> QKTGTAEMSSILEERILGADTSVDLEETGRVLSIGDGIARVHGLRNVQAEEMVEFSSGLKGMSLNLEPDNVGVVVFGNDKLIKEGDIVKRTGAIVDVPVGDELLGRVVDALGNAIDGKGPVGSKIRRRVGLKAPGIIPRISVREPMQTGIKAVDSLVPIGRGQRELIIGDRQTGKTSIAIDTIINQKRFNDGTDEKKKLYCIYVAIGQKRSTVAQLVKRLTDADAMKYTIVVSATASDAAPLQYLAPYSGCSMGEYFRDNGKHALIIYDDLSKQAVAYRQMSLLLRRPPGREAYPGDVFYLHSRLLERAAKMNDSFGGGSLTALPVIETQAGDVSAYIPTNVISITDGQIFLETELFYKGIRPAINVGLSVSRVGSAAQTRAMKQVAGTMKLELAQYREVAAFAQFGSDLDAATQQLLSRGVRLTELLKQGQYSPMAIEEQVAVIYAGVRGYLDKLEPSKITKFESAFLSHVV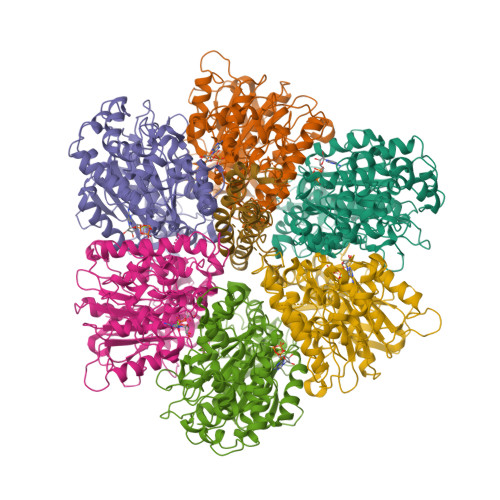SQHQSLLGNIRSDGKISEQSDAKLKEIVTNFLAGFEP;> SAAPKAGTATGQIVAVIGAVVDVQFDEGLPPILNALEVQGRESRLVLEVAQHLGESTVRTIAMDGTEGLVRGQKVLDSGAPIKIPVGPETLGRIMNVIGEPIDERGPIKTKQFAPIHAEAPEFIEMSVEQEILVTGIKVVDLLAPYAKGGKIGLFGGAGVGKTVLIMELINNVAKAHGGYSVFAGVGERTREGNDLYHEMIESGVINLKDATSKVALVYGQMNEPPGARARVALTGLTVAEYFRDQEGQDVLLFIDNIFRFTQAGSEVSALLGRIPSAVGYQPTLATDMGTMQERITTTKKGSITSVQAIYVPADDLTDPAPATTFAHLDATTVLSRAIAELGIYPAVDPLDSTSRIMDPNIVGSEHYDVARGVQKILQDYKSLQDIIAILGMDELSEEDKLTVSRARKIQRFLSQPFQVAEVFTGHMGKLVPLKETIKGFQQILAGDYDHLPEQAFYMVGPIEEAVAKADKLAEEHGS;> ATLKDITRRLKSIKNIQKITKSMKMVAAAKYARAERELKPARVYGTGSLALYEKAEIKGPEDKKKHLIIGVSSDRGLCGAIHSSVAKQMKNDMAALTAAGKEVMIVGIGEKIKSILYRTHSDQFLVSFKDVGRKPPTFGDASVIALELLNSGYEFDEGSIIFNQFKSVISYKTEEKPIFSFSTVVAAENMSIYDDIDADVLQNYQEYNLANIIYYSLKESTTSEQSARMTAMDNASKNASDMIDKLTLTFNRTRQAVITKELIEIISGAAALD2-SUCCINYLBENZOATE | C11 H10 O5 | 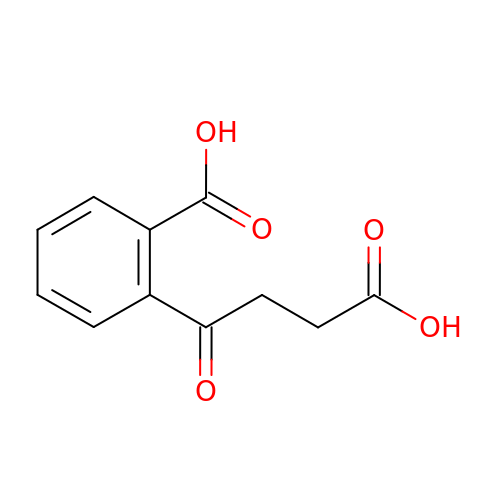YIVWQNVQRXFZJB-UHFFFAOYSA-N> GSGQMFGNGKGSYFITSKDNETGITGIRVFVGPVGLIKSIQVRYGSSWSEKYGIPGGKAHELILHPGEHIISIYGRYRTFLQHVTLITNQGR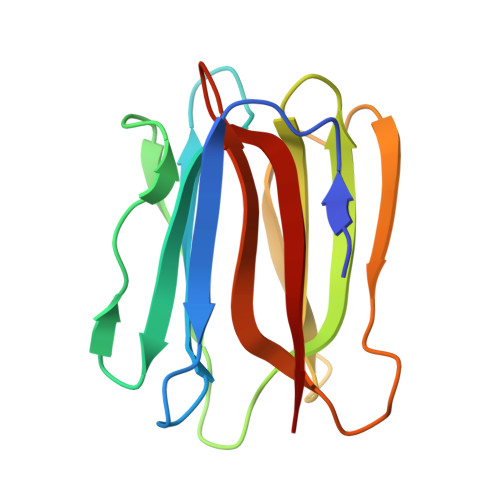SASFGLETGKGFFAAPNLTGQVLEGVYGQFWLYGITGIGFTWGF> GSDSAITLWQFLLQLLQKPQNKHMICWTSNDGQFKLLQAEEVARLWGIRKNK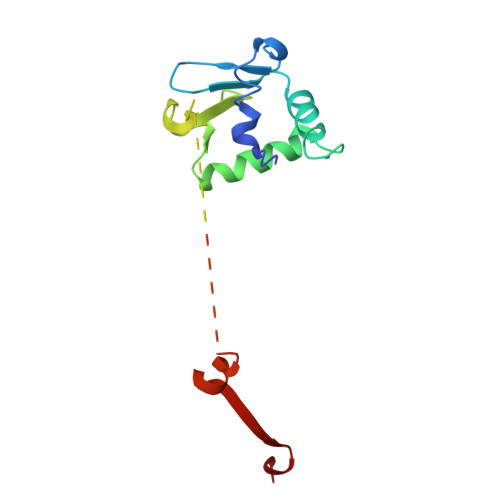PNMNYDKLSRALRYYYVKNIIKKVNGQKFVYKFVSYPEILNMDPMTVGRIEGDCESLNFSEVSSSSKDVENGGKDKPPQPGAKTSSRNDYIHSGLYSSFTLNSLN>MSDTSPGPEHAPAIDRLLQIATGFMASKVLLVAASLGLFTELAAGPLRGEELRARLRLHPRSARDFFDTLVALGVLERTNGAYANTPATAQYLVRGKSAYLGGLLEMSDARMYELWGRLDEGLRTGNPQNEIRTGEEGIYATLYDDPDRLDAFQQAMTGLSMRSAHALAEAIDWSAYRTVADIGCAEGTVLIHLLERHPHLRGTGFDLAAVRPSFQRRHEESGLGDRLAFRAGDFFAEPLPQADALVFGHILSNWALPKAKTLLRKAHEALPEGGIVVIYETLIDDERRENVPGLLMSLTMLLETPGGFEYTGADCREWLADAGFRESRVQYLAGPESMVIATK[2x]

Among bisindoles, reductasporine is distinct due to its dimethylpyrrolinium structure. Its previously reported biosynthetic gene cluster encodes two unique tailoring enzymes, the imine reductase RedE and the dimethyltransferase RedM, which were shown to produce reductasporine from a common bisindole intermediate in recombinant E. coli. RedE reduces compound 4 to didemethylreductasporine, and then RedM catalyzes two methylations to give reductasporine. RedM is a homodimeric protein with monomers consisting of a largely α-helical N-terminal domain (α1-10, β1-3) and a Rossmann-like fold C-terminal domain (α12–16, β4-10) bridged by a long interdomain α-helix (α11). The C-terminal domain possesses a Rossmann-like fold typical of Class I SAM-dependent methyltransferases, with a β-sheet of five parallel strands terminated with two antiparallel strands each interspersed with α-helices.

To provide insight into the N,N-dimethylation catalyzed by RedM, we solved the structure of selenomethionine-labeled RedM, and used this model to solve crystal structures of unliganded enzyme, as well as a co-crystal structure with SAH and a co-crystal structure with SAM, all to 1.7 to 1.85 Å resolution. The homodimers of both unliganded-RedM and RedM-SAH structures superpose well on each other (rmsdCα = 0.175 Å, 553 Cα) and comparatively poorly upon the RedM-SAM homodimer (rmsdCα = 1.244 Å, 593 Cα) due to a substantial displacement of the C-terminal Rossmann-like SAM-binding domain. Lastly, Chain B of the RedM-SAH complex and unliganded-RedM chain A have slightly rotated Rossman-like domains compared to their dimer partners with an average Cα displacement of 1.8 Å between each pair. The two domains of each monomer are separated by a gap of ∼12 amino acids between residues ∼132 and ∼144 ahead of the long interdomain α-helix (α11), which lacks clear electron density in each structure. Each RedM structure has a disordered region around residues 133 to 149, which includes the analogous position (Y140).> GDPVEDIIHDALGNTARRAISGATNVESAADTTPSSHRLETGRVPALQAAETGATSNATDENMIETRCVINRNGVLETTINHFFSRSGLVGVVNLTDGGDTTGYATWDIDIMGFVQLRRKCEMFTYMRFNAEFTFVTTTKSGEARPYMLQYMYVPPGAPKPTGRDAFQWQTATNPSVFVKLTDPPAQVSVPFMSPASAYQWFYDGYPTFGQHPETSNTTYGLCPNNMMGTFAVRVVSREASQLKLQTRVYMKLKHVRAWVPRPIRSQPYLLKNFPNYDSSKITNSARDRSSIKQANM;> MGAQVSTQKSGSHETGNVATGGSTINFTNINYYKDSYAASATRQDFTQDPKKFTQPVLDSIRELSAPLNSPSVEACGYSDRVAQLTVGNSSITTQEAANIVLAYGEWPEYCPDTDATAVDKPTRPDVSVNRFYTLDSKMWQENSTGWYWKFPDVLNKTGVFGQNAQFHYLYRSGFCLHVQCNASKFHQGALLVAVIPEFVIAGRGSNTKPNEAPHPGFTTTFPGTTGATFHDPYVLDSGVPLSQALIYPHQWVNLRTNNCATVIVPYINAVPFDSAINHSNFGLVVVPVSPLKYSSGATTAIPITITIAPLNSEFGGLRQAVSQ;> GIPAELRPGTNQFLTTDDDTAAPILPGFTPTPTIHIPGEVHSLLELCRVETILEVNNTTEATGLTRLLIPVSSQNKADELCAAFMVDPGRIGPWQSTLV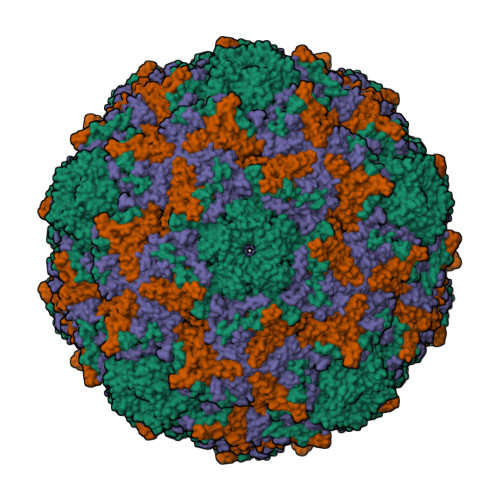GQICRYYTQWSGSLKVTFMFTGSFMATGKMLVAYSPPGSAQPANRETAMLGTHVIWDFGLQSSVSLVIPWISNTHFRTAKTGGNYDYYTAGVVTLWYQTNYVVPPETPGEAYIIAMGAAQDNFTLKICKDTDEVTQQAVLQ> PNFSGNWKIIRSENFEELLKVLGVNVMLRKIAVAAASKYAVEIKQEGD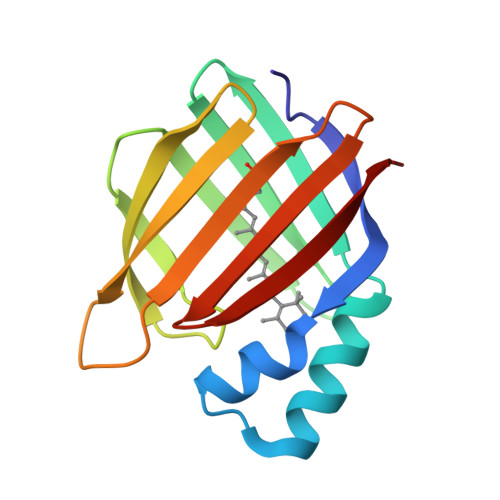TFYIKVSTTVYTTEINFKVGEEFEEQTVDGRPCKSLVKWESENKMVCEQKLLKGEGPKTSWTKELTNDGELILTMTADDVVCTQVFVRE>[2x]MNDFHRDTWAEVDLDAIYDNVENLRRLLPDDTHIMAVVKANAYGHGDVQVARTALEAGASRLAVAFLDEALALREKGIEAPILVLGASRPADAALAAQQRIALTVFRSDWLEEASALYSGPFPIHFHLKMDTGMGRLGVKDEEETKRIVALIERHPHFVLEGLYTHFATADEVNTDYFSYQYTR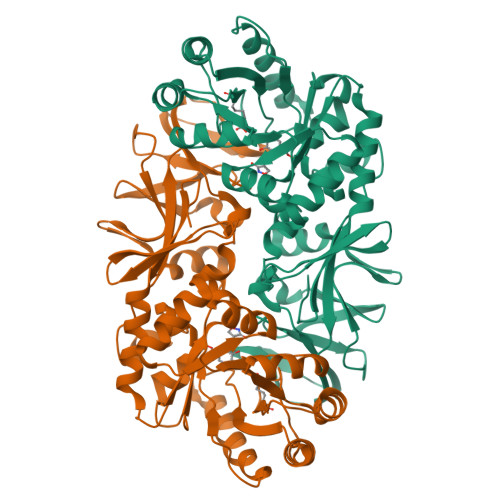FLHMLEWLPSRPPLVHCANSAASLRFPDRTFNMVRFGIAMYGLAPSPGIKPLLPYPLKEAFSLHSRLVHVKKLQPGEKVSYGATYTAQTEEWIGTIPIGYADGWLRRLQHFHVLVDGQKAPIVGRICMDQCMIRLPGPLPVGTKVTLIGRQGDEVISIDDVARHLETINYEVPCTISYRVPRIFFRHKRIMEVRNAIGRGESSA> EEDDGDVA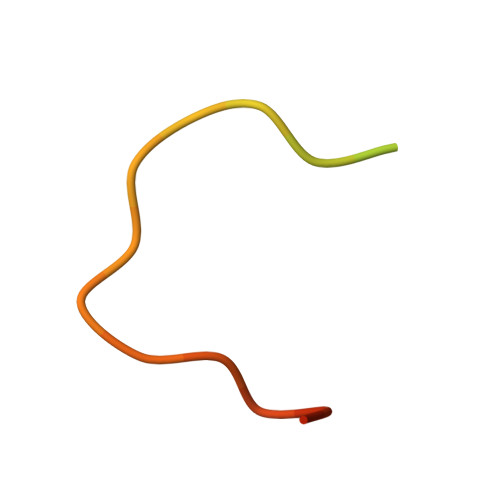MSDAQDGPRVRYNPYTTRPNRR> GCC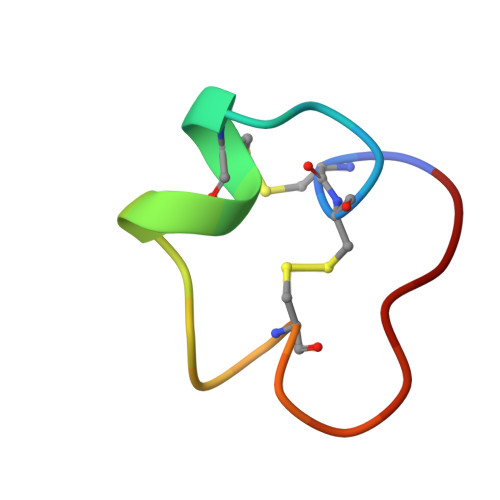SDPRCNYDHPEICGGAAGG> QGPLGSSKVSEQLKCCSGILKEMFAKKHAAYAWPFYKPVDVEALGLHDYCDIIKHPMDMSTIKSKLEAREYRDAQEFGADVRLMFSNCYKYNPPDHEVVA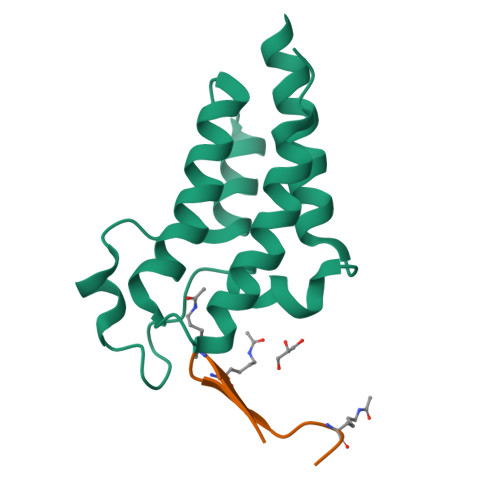MARKLQDVFEMRFAKMPDEPEEP;> XWKTIKGKTWRTKQC>MIIGYARVSSLDQNLERQLENLKTFGAEKIFTEKQSGKSIENRPILQKA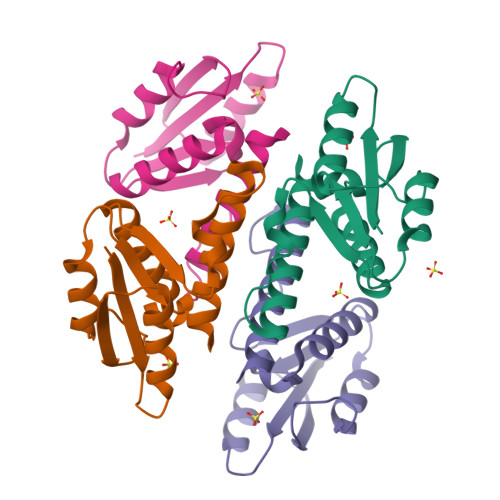LNFVEMGDRFIVESIDRLGRNYNEVIHTVNYLKDKEVQLMITSLPMMNEVIGNPLLDKFMKDLIIRILAMVSEQE[12x]>GAMGSRLYDRRSIFDAVAQSNCQELESLLPFLQRSKKRLTDSEFKDPETGKTCLLKAMLNLHNGQNDTIALLLDVARKTDSLKQFVNASYTDSYYKGQTALHIAIERRNMTLVTLLVENGADVQAAANGDFFKKTKGRPGFYFGELPLSLAACTNQLAIVKFLLQNSWQPADISARDSVGNTVLHALVEVADNTVDNTKFVTSMYNEILILGAKLHPTLKLEEITNRKGLTPLALAASSGKIGVLAYILQREIHEPECRHLSRKFTEWAYGPVHSSLYDLSCIDTCEKNSVLEVIAYSSSETPNRHDMLLVEPLNRLLQDKWDRFVKRIFYFNFFVYCLYMIIFTAAAYYRPVEGLPPYKLKNTVGDYFRVTGEILSVSGGVYFFFRGIQYFLQRRPSLKSLFVDSYSEILFFVQSLFMLVSVVLYFSQRKEYVASMVFSLAMGWTNMLYYTRGFQQMGIYAVMIEKMILRDLCRFMFVYLVFLF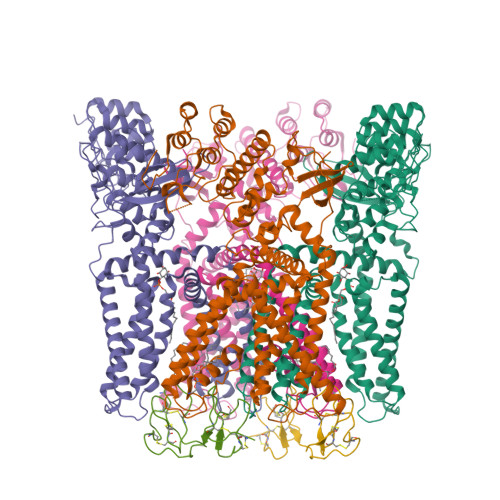GFSTAVVTLIEDGKYNSLYSTCLELFKFTIGMGDLEFTENYDFKAVFIILLLAYVILTYILLLNMLIALMGETVNKIAQESKNIWKLQRAITILDTEKSFLKCMRKAFRSGKLLQVGFTPDGKDDYRWCFRVDEVNWTTWNTNVGIINEDPG[4x];>[2x]MDCAKEGEVCSWGKKCCDLDNFYCPMEFIPHCKKYKPYVPVTTNCAKEGEVCGWGSKCCHGLDCPLAFIPYCEKYR> ASVKDTYTDRLDDWNGIIAGNQYYDSKNDQMAKLNQELEGKVADSLSSISSQADRIYLWEKFSNYKTSANLTATYRKLEEMAKQVTNPSSRYYQDETVVRTVRDSMEWMHKHVYNSEKSIVGNWWDYEIGTPRAINNTLSLMKEYFSDEEIKKYTDVIEKFVPDPEHFRKTTDNPFKALGGNLVDMGRVKVIAGLLRKDDQEISSTIRSIEQVFKLVDQGEGFYQDGSYIDHTNVAYTGAFGNVLIDGLSQLLPVIQKTKNPIDKDKMQTMYHWIDKSFAPLLVNGELMDMSRGRSISRANSEGHVAAVEVLRGIHRIADMSEGETKQRLQSLVKTIVQSD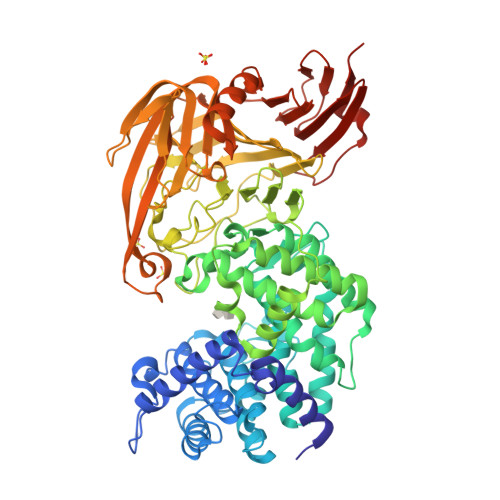SYYDVFKNLKTYKDISLMQSLLSDAGVASVPRTSYLSAFNKMDKTAMYNAEKGFGFGLSLFSSRTLNYEHMNKENKRGWYTSDGMFYLYNGDLSHYSDGYWPTVNPYKMPGTTETDAKRADSDTGKVLPSAFVGTSKLDDANATATMDFTNWNQTLTAHKSWFMLKDKIAFLGSNIQNTSTDTAATTIDQRKLESSNPYKVYVNDKEASLTEQEKDYPETQSVFLESSDSKKNIGYFFFKKSSISMSKALQKGAWKDINEGQSDKEVENEFLTISQAHKQNGDSYGYMLIPNVDRATFNQMIKELESSLIENNETLQSVYDAKQGVWGIVKYDDSVSTISNQFQVLKRGVYTIRKEGDEYKIAYYNPETQESAPDQEVFKKLEQHHHHHH> MKPTIPPDDSDTAGKQVEVEKENETIQELMIALQIHSGYTNISYT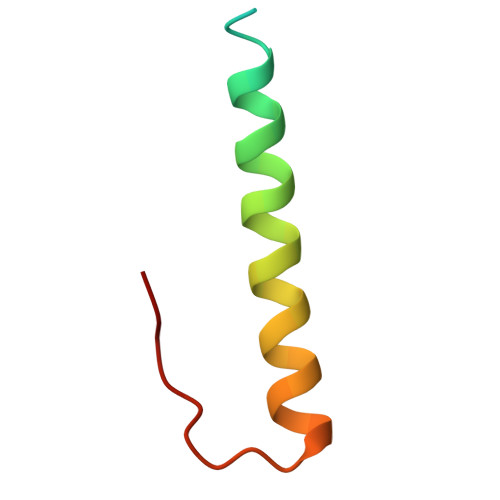I>MGRILVIEDEISLNKTIIDNLNEFGYQTDSSENFKDGEYFIGIRHYDLVLASWNLPDGDGAELVNTIKHKSPRTSVMIMSAKADKDTEIKALKAGADDFVKKPLDFDILLARIEARLRLGGTNVIKIEDLVIDPDEEKITYKGQDIELKGKPFEVLTHLA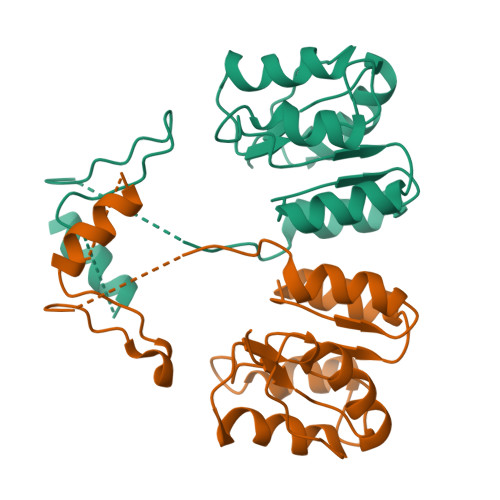RHSDQIVSKEQLLDAIWEEPELVTPNVIEVAINQIRQKMDKPLNISTIETVRRRGYRFCFPKKS[2x]>GMSGTANSRRKEVLRVPVIDLNRVSDEEQLLPVVRAILLQHDTFLLKNYANKAVLDALLAGLTTKDLPDTSQGFDANFTGTLPLEDDVWLEQYIFDTDPQLRFDRKCRNESLCSIYSRLFKLGLFFAQLCVKSVVSSAELQDCISTSHYATKLTRYFNDNGSTHDGADAGATVLPTGDDFQYLFERDYVTFLPTGVLTIFPCAKAIRYKPSTMATTDNSWVSIDEPDCLLFHTGTLLARWSQGMHTTSPLQIDPRANIVSLTIWPPLTTPISSKGEGTIANHLLEQQIKAFPKVAQQYYPRELSILRLQDAMKFVKELFTVCETVLSLNALSRSTGVPPELHVLLPQISSMMKRKIVQDDILKLLTIWSDAYVVELNSRGELTMNLPKRDNLTTLTNKSRTLAFVERAESWYQQVIAS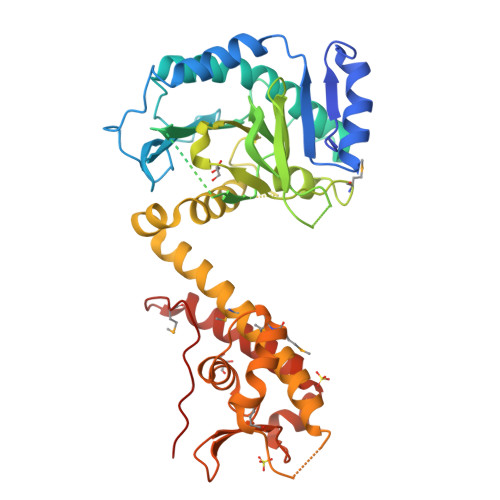KDEIMTDVPAFKINKRRSSSN[3x]> MTAKDDYPSLSFQQDYVYIFSSDFQLSEELGVALINALSAKEIVPERLYVMLNDKTISFSFISKNKKSKNRVLSTEKKLNYKHISEYIVNEIEY;> MGSSHHHHHHSQDPVHFYETSYKYQAADSTYMHDVAINVSIKGNHFTSDIIIRELVKSENKNYYNVIGHGDIIQKNTHQYYLNFDNIDVYTGTNKANMKPYKEPTSISSLINKSNNIRVVYLSEEYVVVEFFFYDGQIITLHRY

In V. parahaemolyticus, the activation of T3SS2 by bile salts is regulated by two transmembrane ToxR-like transcription factors, VtrA (VPA1332) and VtrB (VPA1348). Furthermore, we demonstrate that the periplasmic domains of the transmembrane proteins, VtrA and VtrC, form a functional complex that binds bile salts to activate VtrA’s cytoplasmic DNA binding domain, which in turn induces T3SS2 via the downstream transcription factor VtrB. The structure of VtrA/VtrC periplasmic domains reveals an obligate heterodimer where VtrC recruits structural elements from VtrA to complete a β-barrel with a hydrophobic inner chamber that binds bile salts. Our biochemical data and the structural analysis demonstrated that the periplasmic domains of the inner membrane proteins VtrA and VtrC form a stable complex that functions as a receptor for bile salts.

To further understand the nature of the interaction between the periplasmic domains of VtrA and VtrC, we crystallized the complex and obtained its X-ray structure. The structure was solved by multiple-wavelength anomalous dispersion phasing using anomalous signals from selenomethionine and refined to a resolution of 2.70 Å using native data from an isomorphous crystal. The asymmetric unit contains one complex with one copy each of the VtrC and VtrA periplasmic domains. The VtrA and VtrC subunits in the heterodimer make extensive interactions with each other, with an interface area of 1,149 Å2. The VtrC subunit consists of eight β-strands and a short α-helix. The eight β-strands of VtrC form a β-sheet meander that folds into itself to form a β-barrel with a small space between the first and last β-strands (Aβ and Iβ). The β-barrel is lined on the inside by hydrophobic side chains and is covered on one side by the short α-helix (Fα) and an adjacent disordered loop, which could not be modeled in its entirety due to the poor electron density of this region. The Hβ-Iβ loop is particularly rich in aromatic side-chains, promoting us to hypothesize that this loop could be involved in binding the steroid ring structure of bile acids. VtrA Fβ intercalates between VtrC Aβ and Iβ, making numerous polar contacts with VtrC Aβ and closing the gap in the VtrC β-barrel. The incorporation of structural elements from VtrA into the β-barrel fold suggests that VtrC may not fold properly in isolation and is consistent with our inability to purify the VtrC periplasmic domain in the absence of VtrA.5-(5-hydroxyl-isoxazol-3-yl)-furan-2-phosphonic 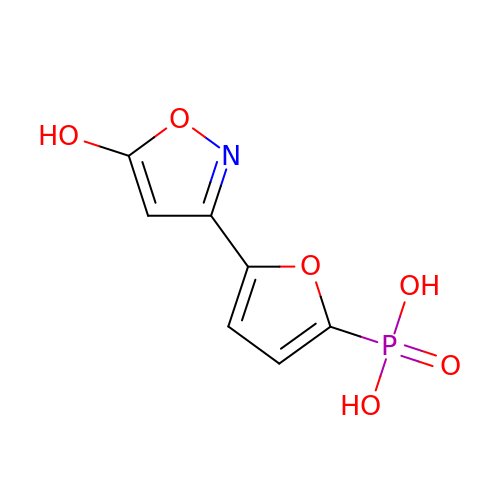acid | C7 H6 N O6 P | BRLJHMCTDKAUAY-UHFFFAOYSA-N>[3x]MEVRKVIAAGEVIESPVDVVKELVENSLDAKATKVEVEIVKGGKRLIRVKDNGTGIHPEDVEKVVLQGATSKIETEKDLMNISTYGFRGEALYSISSVSKFKLRSRFFQEKEGKE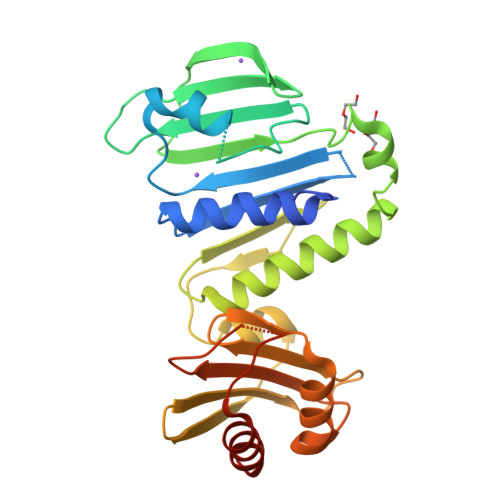IEVEAGNILGTRRVGMPVGTEVEVRDLFFNLPVRRKFLKKEDTERRKVLELIKEYALTNPEVEFTLFSEGRETLKLKKSSLKERVEEVFQTKTEELYAEREGITLRAFVSRNQRQGKYYVFINKRPIQNNNLKEFLRKVFGYKTLVVLYAELPPFMVDFNVHPKKKEVNILKERKFLELVRELAGKEKPIVDI>AGAGAAGAUCUUCUCU[6x]

Since DNA/RNA duplexes are known to be less stable than RNA/RNA duplexes, we have examined the impact of dA, dI, and dG substitutions on RNA structure and nonenzymatic template copying. In this study, we have investigated the effects of 2′-deoxyribo-purines on nonenzymatic template copying by conducting thermodynamic, structural, and kinetic analyses. Structural analyses of RNA duplexes containing 2′-deoxyribo-purine nucleotides suggest that the observed destabilization is likely due to reduced solvation effects, since base pairing and sugar conformations are unchanged. Our results suggest that a primordial genetic polymer containing both ribo- and 2′-deoxyribo- nucleotides would likely behave similarly to RNA but with somewhat slower template copying chemistry, offset by a possible advantage in strand separation and exchange, which could in turn facilitate cycles of replication.

Among these, four sequences (dAU1, dAU2, dAUS1, and dAUS2) contained base pairs involving deoxyadenosine (dA:U and dA:s2U), four (dGC1, dGC2, dGCS1, and dGCS2) contained deoxyguanosine base pairs (dG:C and dG:s2C), and two (dICS1 and dICS2) included base pairs with deoxyinosine (dI:s2C). In contrast, sequences containing dG:s2C formed distinct crystal lattices. The dGCS2 duplex crystallized in space group P31, with six strands per unit cell. Notably, sequences containing dG:s2C pairs crystallized in a distinct lattice from the same sequence with G:s2C pairs, which may reflect a markedly increased flexibility in dG sugar pucker conformation compared to dA or dI. This interpretation is consistent with thermodynamic data showing a greater entropic penalty associated with replacing rG with dG. In some other cases, likely due to changes in crystal packing, Water 1 is not visible, for example at the dG7 position in dGCS2, in contrast to its clear presence at G7 in GCS2. However, in the case of dG7 in the dGCS2 structure, altered crystal packing prevents Water 2 from forming hydrogen bonds with either Water 3 or nonbridging phosphate oxygens. In contrast, base pairs involving deoxyguanosine (dG) display enthalpic gains but entropic penalties compared to their G-containing counterparts. The net ΔG°25°C penalty for base pairs with dG is ~0.5–0.6 kcal/mol.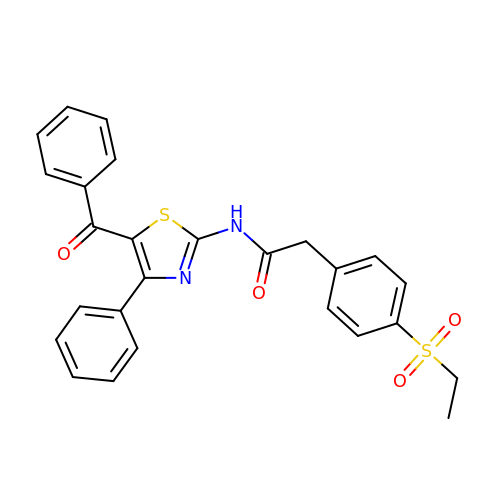2-(4-ethylsulfonylphenyl)-~{N}-[4-phenyl-5-(phenylcarbonyl)-1,3-thiazol-2-yl]ethanamide | C26 H22 N2 O4 S2 | MDMLFHGEDDZHNU-UHFFFAOYSA-N> MSSPINDYFIDYNPLFPIFATRIAKGLAIYRVSDHARLAVIPIRNINLVANYDWDTTTGKFLSIFFKDGTIRIHDIFKDGRLVSFLRIPSTKISKGIWDRIPLRYEPNNRDFACNIIDDLPKLIRFVKDSKRINIVPYTQPNSLWRGPDEDDLDSNEKLDVHVVFNEGNDKITVFFNGDYAVFLSVDNIENENSLKSIIKVQDGFYQCFYEDGTVQTLNLGPLLQSKSSVNLLNYIMVIKELIGYMLTHLEFINRELATPYLDFVKRLCDEAYGYGKLKSELEALFLLGEISCDLEDWLCNSVGEKNFKRWKYLGCEAYQKTVQILTLIFVPACERIIIYVEKLRAILQAFSIQNKLSYTSDLTAVEVLLKSSQKLLTMTLNSIIGLGRDETLFEKFFIWFNDRLHEALDEDYKLKFQFEDDLYFGYDLLSYFDRILSKKGTEPSSIIDVKLYRDLINSMSDMEKDIAQSNVNSHIQQHILVDLKTDVFAQKYPSSQINLLDAIKLPKHNYIVYLIQVTKHNSAQEPFSEENKKKLYIGTLKDENLGIISKESSVKIPALFKSYRLSSTRFVPNRVHSLLRDIGLSDSNYHSSHVTDYRGENYENEEDDGTIAIPAYIREN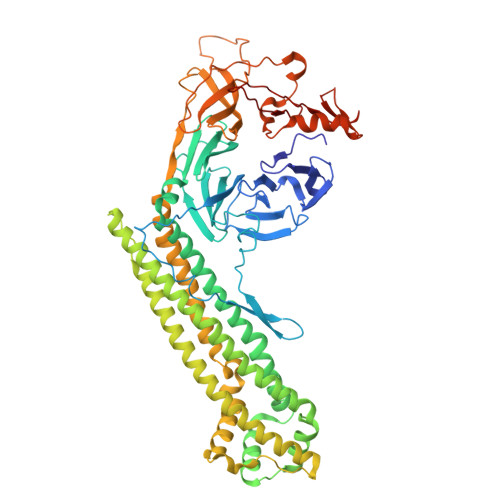RENDDFIACTAKVSVDGRSASLVFPKEKQNV>DYKDDDDKLHSQANLMRLKSDLFNRSPMYPGPTKDDPLTVTLGFTLQDIVKADSSTNEVDLVYWEQQRWKLNSLMWDPNEYGNITDFRTSAADIWTPDITAYSSTRPVQVLSPQIAVVTHDGSVMFIPAQRLSFMCDPTGVDSEEGATCAVKFGSWVYSGFEIDLKTDTDQVDLSSYYASSKYEILSATQTRQVQHYSCCPEPYIDVN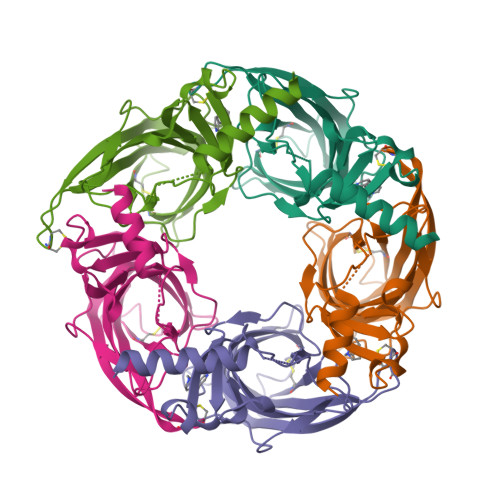LVVKFRERRAGNGFFRNLFDSR[5x]>MPLNRTLEMSELPGLEDWEDEFDLENAVLFEVAWEVANKVGGIYTVLQTKAKVTGDEWGDNYFLVGPYTEQGVRTQVELLEAPTPALKRTLDSMNSKGCKVYFGRWLIEGGPLVVLLDVGASAWALERWKGELWDTCNIGVPWYDREANDAVLFGFLTTWFLGEFLAQSEEKPHVVAHFHEWLAGVGLCLCRARRLPVATIFTTHATLLGRYLCAGAVDFYNNLENFNVDKEAGERQIYHRYCMERAAAHCAHVFTTVSQITAIEAQHLLKRKPDIVTPNGLNVKKFSAMHEFQNLHAQSKARIQEFVRGHFYGHLDFNLDKTLYFFIAGRYEFSNKGADVFLEALARLNYLLRVNGSEQTVVAFFIMPARTNNFNVETLKGQAVRKQLWDTANTVKEKFGRKLYESLLVGSLPDMNKMLDKEDFTMMKRAIFATQRQSFPPVCTHNMLDDSSDPILTTIRRIGLFNSSADRVKVIFHPEFLSSTSPLLPVDYEEFVRGCHLGVFPSYYEPWGYTPAECTVMGIPSISTNLSGFGCFMEEHIADPSAYGIYILDRRFRSLDDSCSQLTSFLYSFCQQSRRQRIIQRNRTERLSDLLDWKYLGRYYMSARHMALSKAFPEHFTYEPNEADAAQGY[4x];>[3x]GPMTDQAFVTLTTNDAYAKGALVLGSSLKQHRTTRRLVVLATPQVSDSMRKVLETVFDEVIMVDVLDSGDSAHLTLMKRPELGVTLTKLHCWSLTQYSKCVFMDADTLVLANIDDLFDREELSAAPDPGWPDCFNSGVFVYQPSVETYNQLLHLASEQGSFDGGDQGILNTFFSSWATTDIRKHLPFIYNLSSISIFSYLPAFKVFGASAKVVHFLGRVKPWNYTYDPKTKSVKSEAHDPNMTHPEFLILWWNIFTTNVLPLLQQFGLVKDTCSYVNVLSDLVYTLAFSCGFCRKEDVSGAI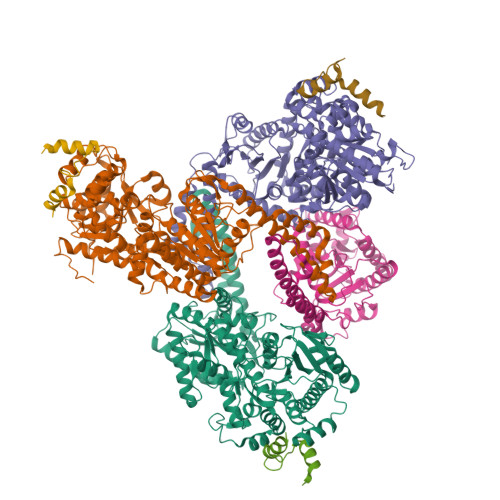SHLSLGEIPAMAQPFVSSEERKERWEQGQADYMGADSFDNIKRKLDTYLQ>[4x]MNAPESVQAKPRKRYDAGVMKYKMGYWDGDYVPKDTDLLALFRITPQDGVDPVEAAAAVAGESSTATWTVVWTDRLTACDMYRAKAYRVDPVPNNPEQFFCYVAYDLSLFEEGSIANLTASIIGNVFSFKPIKAARLEDMRFPVAYVKTFAGPSTGIIVERERLDKFGRPLLGATTKPKLGLSGRNYGRVVYEGLKGGLDFMKDDENINSQPFMHWRDRFLFVMDAVNKASAATGEVKGSYLNVTAGTMEEMYRRAEFAKSLGSVIIMVDLIVGWTCIQSMSNWCRQNDMILHLHRAGHGTYTRQKNHGVSFRVIAKWLRLAGVDHMHTGTAVGKLEGDPLTVQGYYNVCRDAYTQTDLTRGLFFDQDWASLRKVMPVASGGIHAGQMHQLIHLFGDDVVLQFGGGTIGHPQGIQAGATANRVALEAMVLARNEGRDILNEGPEILRDAARWCGPLRAALDTWGDISFNYTPTDTSDFAPTASVA;>[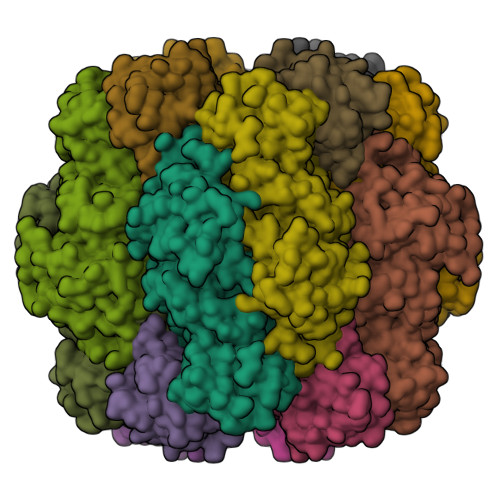4x]MRITQGTFSFLPELTDEQITKQLEYCLNQGWAVGLEYTDDPHPRNTYWEMFGLPMFDLRDAAGILMEINNARNTFPNHYIRVTAFDSTHTVESVVMSFIVNRPADEPGFRLVRQEEPGRTLRYSIESYAVQAGPEGSRY>MEVVKFMDVYQRSYCHPIETLVDIFQEYPDEIEYIFKPSCVPLMRCGGCCNDEGLECVPTEESNITMQIMRIKPHQGQHIGEMSFLQHNKCECRPK[2x]

In the present work, we focus on a class of monocyclic disulfide‐containing 19 amino acid peptides targeting the Vascular Endothelial Growth Factor‐A, the main pro‐angiogenic factor in Human. We proposed to use this peptide as a model to rationalize the thermodynamics of α‐helix stabilization by an i to i+4 lactam bridge. Around 950 Å2 of accessible surface area (ASA) was buried at the peptide‐VEGF interface, that overlapped with the VEGF receptor 1 domain 2 (VEGFR1‐d2)‐binding site. Although only lactam‐bridged ExxxK, DxxxK and KxxxD induced the formation of stable helix in the unbound state, all peptides of the series were helically folded when bound to VEGF.

VEGF‐peptide 2 c mixture crystallized also in a tetragonal form that contained no bound peptide. The main backbone displacements occurred in the 83–89 and 35–46 loops, that are flexible in molecular modelling studies as well. Moreover, the conformational exchange involving the flipping of the ϕ dihedral angle of VEGF Asn W62 was already noticed in several crystal structures of apo‐VEGF, which assumes that the two conformations are in dynamical equilibrium in solution.>MFNLPPGNYKKPKLLYCSNGGHFLRILPDGTVDGTRDRSDQHIQLQLSAESVGEVYIKSTETGQYLAMDTDGLLYGSQTPNEECLFLERLEENHYNTYISKKH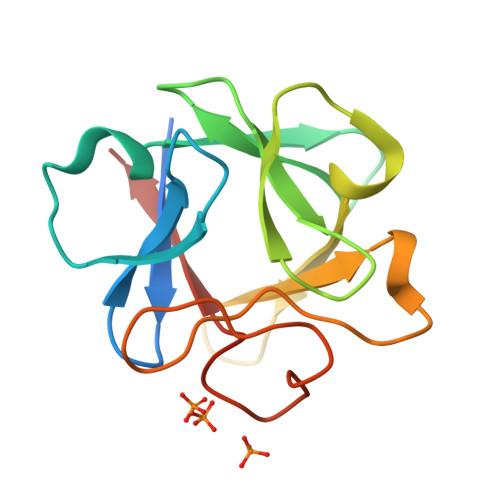AEKNWFVGLKKNGSCKRGPRTHYGQKAILFLPLPVSSD[3x]>[4x]MSSNNSGLSAAGEIDESLYSRQLYVLGKEAMLKMQTSNVLILGLKGLGVEIAKNVVLAGVKSMTVFDPEPVQLADLSTQFFLTEKDIGQKRGDVTRAKLAELNAYVPVNVLDSLDDVTQLSQFQVVVATDTVSLEDKVKINEFCHSSGIRFISSETRGLFGNTFVDLGDEFTVLDPTGEEPRTGMVSDIEPDGTVTMLDDNRHGLEDGNFVRFSEVEGLDKLNDGTLFKVEVLGPFAFRIGSVKEYGEYKKGGIFTEVKVPRKISFKSLKQQLSNPEFVFSDFAKFDRAAQLHLGFQALHQFAVRHNGELPRTMNDEDANELIKLVTDLSVQQPEVLGEGVDVNEDLIKELSYQARGDIPGVVAFFGGLVAQEVLKACSGKFTPLKQFMYFDSLESLPDPKNFPRNEKTTQPVNSRYDNQIAVFGLDFQKKIANSKVFLVGSGAIGCEMLKNWALLGLGSGSDGYIVVTDNDSIEKSNLNRQFLFRPKDVGKNKSEVAAEAVCAMNPDLKGKINAKIDKVGPETEEIFNDSFWESLDFVTNALDNVDARTYVDRRCVFYRKPLLESGTLGTKGNTQVIIPRLTESYSSSRDPPEKSIPLCTLRSFPNKIDHTIAWAKSLFQGYFTDSAENVNMYLTQPNFVEQTLKQSGDVKGVLESISDSLSSKPHNFEDCIKWARLEFEKKFNHDIKQLLFNFPKDAKTSNGEPFWSGAKRAPTPLEFDIYNNDHF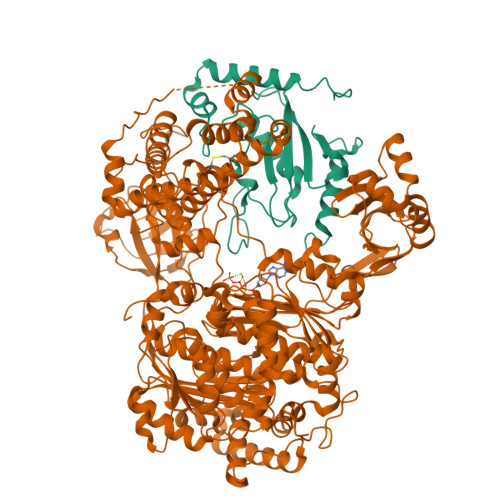HFVVAGASLRAYNYGIKSDDSNSKPNVDEYKSVIDHMIIPEFTPNANLKIQVNDDDPDPNANAANGSDEIDQLVSSLPDPSTLAGFKLEPVDFEKDDDTNHHIEFITACSNCRAQNYFIETADRQKTKFIAGRIIPAIATTTSLVTGLVNLELYKLIDNKTDIEQYKNGFVNLALPFFGFSEPIASPKGEYNNKKYDKIWDRFDIKGDIKLSDLIEHFEKDEGLEITMLSYGVSLLYASFFPPKKLKERLNLPITQLVKLVTKKDIPAHVSTMILEICADDKEGEDVEVPFITIHL;>MSSRKSTASSLLLRQYRELTDPKKAIPSFHIELEDDSNIFTWNIGVMVLNEDSIYHGGFFKAQMRFPEDFPFSPPQFRFTPAIYHPNVYRDGRLCISILHQSGDPMTDEPDAETWSPVQTVESVLISIVSLLEDPNINSPANVDAAVDYRKNPEQYKQRVKMEVERSKQDIPKGFIMPTSESAYISQSKLDEPESNKDMADNFWYDSDLDDDENGSVILQDDDYDDGNNHIPFEDDDVYNYNDNDDDDERIEFEDDDDDDDDSIDNDSVMDRKQPHKAEDESEDVEDVERVSKKI[4x]({[(3E)-2'-OXO-2',7'-DIHYDRO-2,3'-BIINDOL-3(7H)-YLIDENE]AMINO}OXY)ACETIC ACID | C18 H13 N3 O4 | 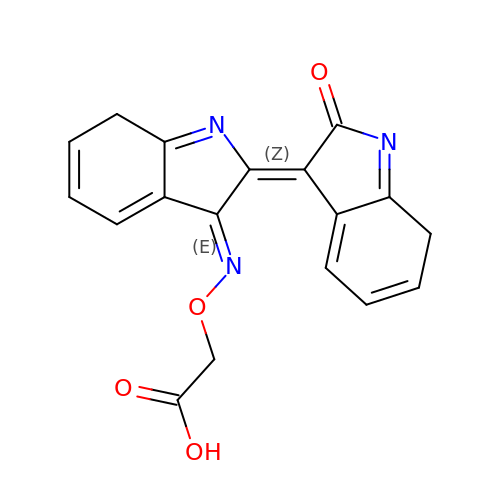BFQRPTKOSYMPOL-LALPNIDTSA-N> MAEEYSWDSYLNDRLLATNQVSGAGLASEEDGVVYA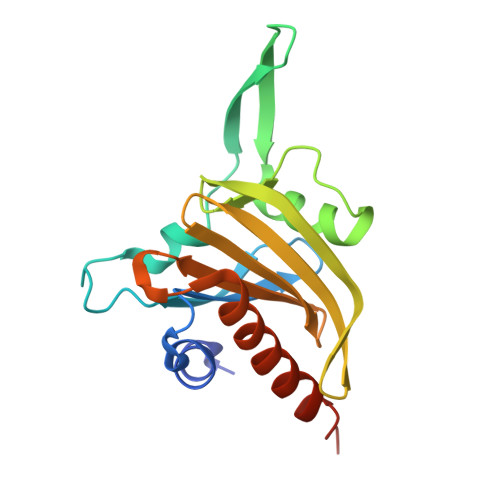CVAQGEESDPNFDKWSLFYKEDYDIEVEDENGTKTTKTINEGQTILVVFNEGYAPDGVWLGGTKYQFINIERDLEFEGYNFDVATCAKLKGGLHLVKVPGGNILVVLYDEEKEQDRGNSKIAALTFAKELAESSQLQHHHHHH> MSRSRPELGDWSSPAELAELQRSQLPRVLAQALRSPFYAARYRGTTPPRTADDFAGVEVTAKQDLRDQYPFGMLAVGREHLATYHESSGTAGEPTASYYTEEDWTDLAERFARKWTGIHPSDTFLVRTPYGLVITGHLAQAAGRLRGATVVPGDARSLATPLSRMVRVLKTLDVTLTWCNPTEITMLAAAAKAAGLRPDQDFPHLRAMFTAAEPLTEVRRRRLSEIWGGIPVVEEYGSTETGTIAGQCPEGRMHLWADRAIFEVYDPRTGTLSEAGRGQMVVTPLYRDAMPLLRYNLADDVEVSTDPCGCGWLLPTVTVLGRAGTGHRIGPATVTQQRLEELVFSLPAAYEVMFWRAKAHPDVLELEFEAPEPVRQRAVKELGAALDRELGVPHRITGLAPGTLVPAEALTAQRDILKARYLFAEDEDWDKAVMYF;> AMSRSRPELGDWSSPAELAELQRSQLPRVLAQALRSPFYAARYRGTTPPRTADDFAGVEVTAKQDLRDQYPFGMLAVGREHLATYHESSGTAGEPTASYYTEEDWTDLAERFARKWTGIHPSDTFLVRTPYGLVITGHLAQAAGRLRGATVVPGDARSLATPLSRMVRVLKTLDVTLTWCNPTEITMLAAAAKAAGLRPDQDFPHLRAMFTAAEPLTEVRRRRLSEIWGGIPVVEEYGSTETGTIAGQCPEGRMHLWADRAIFEVYDPRTGTLSEAGRGQMVVTPLYRDAMPLLRYNLADDVEVSTDPCGCGWLLPTVTVLGRAGTGHRIGPATVTQQRLEELVFSLPAAYEVMFWRAKAHPDVLELEFEAPEPVRQRAVKELGAALDRELGVPHR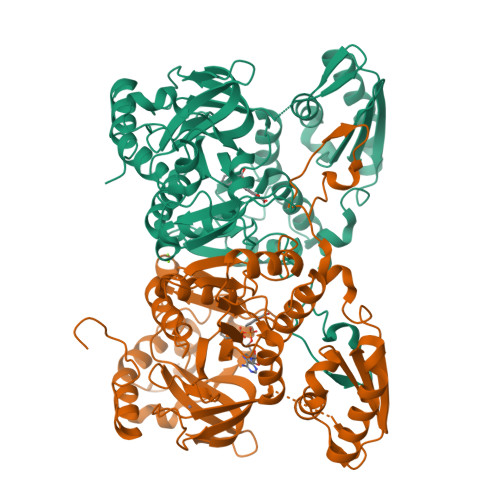ITGLAPGTLVPAEALTAQRDILKARYLFAEDEDWDKAVMYF The two RNA segments in its genome encode four viral proteins, including zinc-binding protein (Z), RNA polymerase (L), nucleoprotein (NP), and the surface glycoprotein precursor (GP, or spike protein). GP is cleaved into envelope glycoproteins GP1 and GP2. GP1 that is responsible for receptor binding (including α-dystroglycan, heparin sulfate, DC-SIGN, etc.) and GP2 that mediates membrane fusion interact with each other to form a stable trimer complex on the LASV viral envelope. The GP2 protein contains a N-terminal fusion peptide (FP) (residues 258-295), a N-terminal HR1 domain (residues 295-363), a linker T-loop domain (residues 363-386), a C-terminal HR2 domain (residues 386-431), a transmembrane domain (residues 431-453), and an intracellular domain (residues 454-491).

To reveal the interaction between HR1 and HR2 domains of LASV, stable 6-HB covering HR1, T-loop and HR2 domains (residues 306–432), was constructed for crystallographic study. After the single mutation of C310S was introduced, the trimeric LASV 6-HB protein was obtained. Then we continued to try different truncations and deletions in 6-HB, and finally found that a deletion of Gly378 and Lys379 in the T-loop region could yield protein crystal with enough quality for structure determination. The overall structure of the HR1-T-loop-HR2 domain showed a canonical 6-HB structure. Taking a rod-like shape with a length of ∼75 Å and a diameter of ∼40 Å, the LASV fusion core contains a parallel trimeric coiled-coil of three HR1 helices (gray in Figure 2A), around which three HR2 helices are entwined (green in Figure 2A) in an antiparallel manner. According to the structure shown in electrostatic potential surface, the HR2 region of LASV can be divided into two parts: a linear N-terminal region and a helical C-terminal region. The linear N-terminal region binds to two adjacent HR1 helices through hydrophobic interactions, consistent with other fusion core structures, as previously determined. Moreover, at the junction region between linear and helical parts of HR2, several strong hydrogen bonds and salt bridges are noted. For salt bridges, Asp402 interacts with Arg325 (∼2.9 Å distance), and Glu404 interacts with Lys320 and Gln324 (∼3.2 Å and 3.6 Å distances, respectively). These relatively concentrated hydrophilic interactions constitute an anchoring point in the middle of HR2 domain, stabilizing the linear and helical region of HR2 and also the whole 6-HB conformation.

> GPHMDEEFSDMLRLFDFNKQAIQRLKAEAQMSIQLINKAVNALINDQLIMKNHLRDIMGIPYCNYSKYWYLNHTTTTSLPKCWLVSNGSYLNETHFSDDIEQQADNMITEMLQKEYMERQGKTPLGLVD2-AMINO-N,3,3-TRIMETHYLBUTANAMIDE 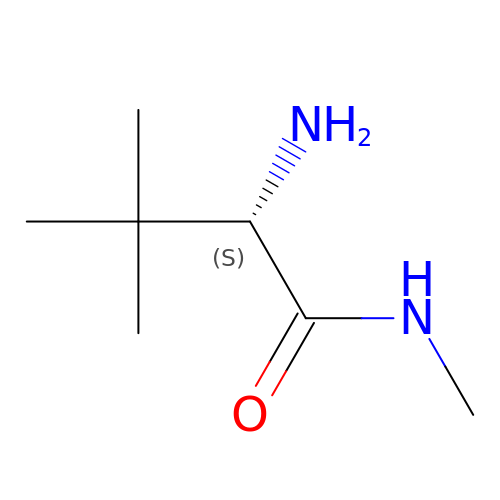| C7 H16 N2 O | BPKJNEIOHOEWLO-RXMQYKEDSA-N> GNHFHVFVGDLSPEITTEDIKAAFAPFGRISDARVVKDMATGKSKGYGFVSFFNKWDAENAIQQMGGQWLGGRQIRTNWA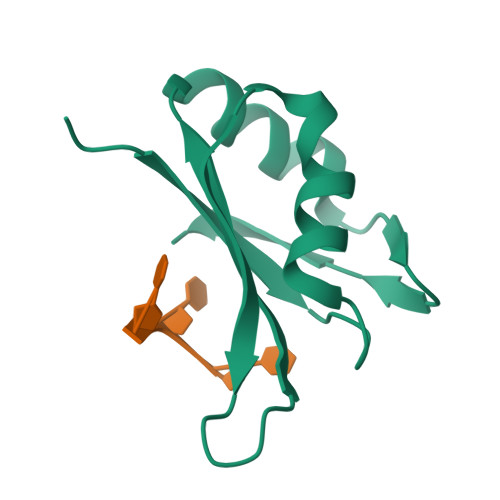TRKPPAPKSTYE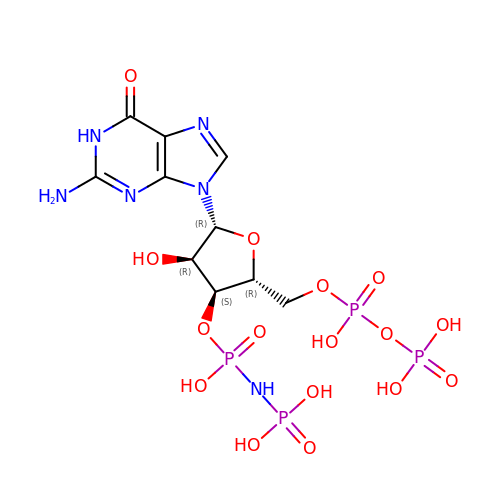[[[(2~{R},3~{S},4~{R},5~{R})-5-(2-azanyl-6-oxidanylidene-1~{H}-purin-9-yl)-4-oxidanyl-2-[[oxidanyl(phosphonooxy)phosphoryl]oxymethyl]oxolan-3-yl]oxy-oxidanyl-phosphoryl]amino]phosphonic acid | C10 H18 N6 O16 P4 | XBDJLYDZMOIGRH-UUOKFMHZSA-N>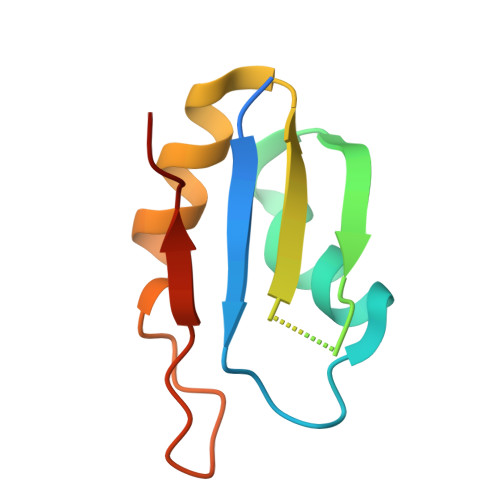 GAGEKAKLFTNVYVKNFTEDFDDEKLKEFFEPYGKITSYKVMSKEDGKSKGFGFVAFETTEAAEAAVQALNGKDMGEGKSLYVARAQKKA>MISGANDPLLDMFFDDDFVPQAFVD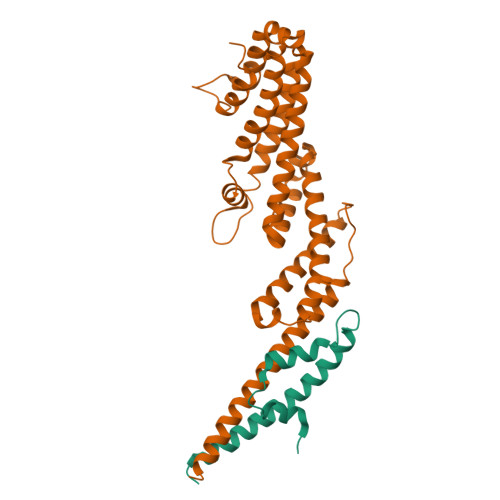ILLSSFQTSQLEELKTNCSSLLSKMDYYSGHITKELESTIQVLQKPAELIIY[2x];>[2x]GSYNRLQQDILEPFERALKLQTVSSKIHQTTTLLRSSLIYVHMISQLQMMPLETDSTDDAALACGLKIAALHSQLKINIAANPNLATLQLIKSCENNVVSPNRQELLRYLSTNLTRDCLNNLKMENNPKRIVTLIKALYTLSPVDLFDTIDKVLSSKIQTTAQVLSKTITSIRNFNLSLDDAMENRNSILTLQNLMAACAIEGNTNTLRNYLSQRKFSSLIDQFWSKVTNSFKRDFEMSYNRGGPVGKSLQSNSNLIYEAISKCFGENDPSNELQGELQYILKAVSILDT N-HYDROXY-4-PHOSPHONO-BUTANAMIDE 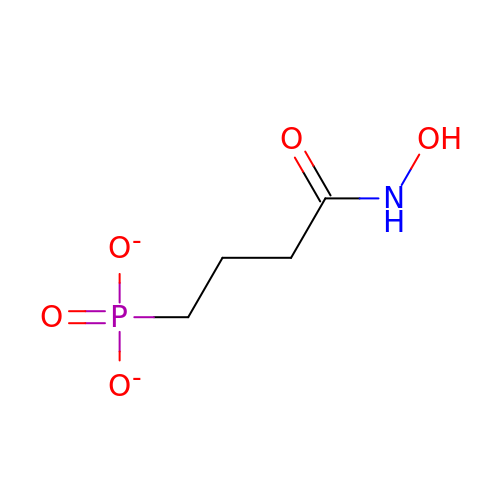| C4 H8 N O5 P | AKXSFRVADDCWTF-UHFFFAOYSA-L> PEP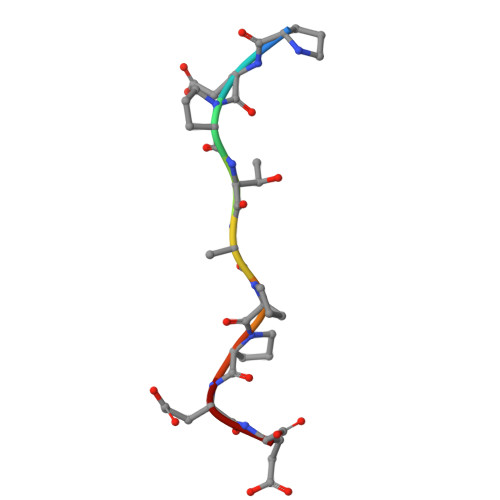TAPPEE> MGSSHHHHHHSSGLVPRGSHMMNTFSSFRKHALLHSKETAVKSINHNISFYNLLLLIQRIATGLKSANIKKGDRISIHMGNCFELIATYYACLKIGAVFVPLSLKLSAKEVKNLIQHSSSCAYIGDKKRFYETKQEIESCTMLEKIWVIDLKIEDKENNTHNWEEIISQPYDYSEDNIYTDEIASIFYTSGTTGHPKGIVYSQKTLIDAVNLTKVTINPRLPKSDGDKPAILSLVDLISPWSILITFAALQKGYSVLLLS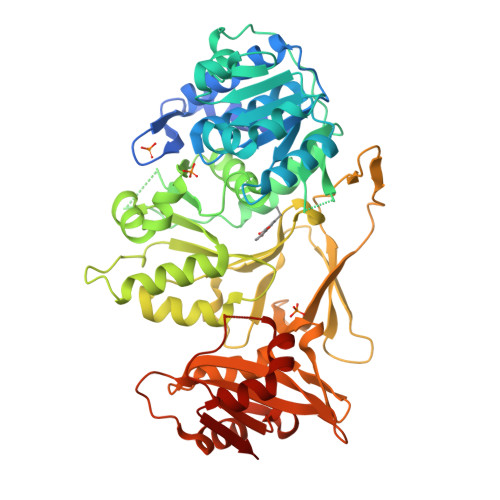EVDIENITETLKETQPAWIAGTPSNFHKIIKNEENNNNSLDLSETVCVAGGDSCATELSQKFFECFGSHLQSSYGQTELGGPVIYHHDIYAINEPSIGWPLPGVEIKINNTQSSNGELLIRSPAKTIGIWNGHDIELFPSDRWLATGDLVRQENNRNLIFLGREKDQIKIEGYPVYPIEIENTLIQHADIAASVVFSVPDKYAGERIIALIQPQKNHSLKAETIASYLSDNLAHYKHPSEYIFIKEIPVNTTGKISRRKLSNEYHLLKSQAEKVFTL5-HYDROXYMETHYLURIDINE-2'-DEOXY-5'-MONOPHOSPHATE | C10 H15 N2 O9 P | 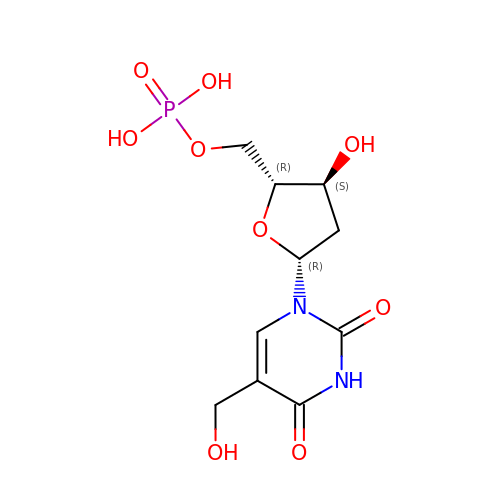WEBVWKFGRVLCNS-XLPZGREQSA-N2',3'-dideoxy-2'-fluoro-3'-triaza-1,2-dien-2-ium-1-yluridine | C9 H11 F N5 O4 | 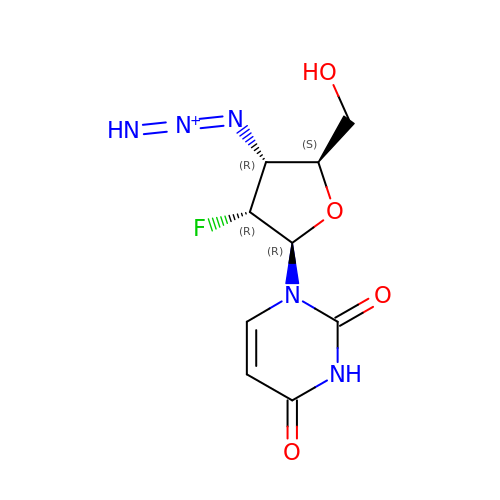YRIDFNZYEULFDH-XVFCMESISA-O>GPEFEAAACKKYMSKLRTIVAAQSRFLSTYDGAENLCLEDIYTENTLEVRTEVGMAGPLHKSPAALGLEELFSPNGHLNEDADTVLVVGEAGSGKSTLLQQVHLLWATGQDFQEFLFVFPFSCRQLQCVARPLSVMTLLFEHCCWPDVGQQDVFQFLLDHPDRILLTFDGFDEFKFKFTDHERHCSPTDPTSVQTLLFNLLQGNLLKNARKVLTSRPDAVSAFLRKYVRTEFNLKGFSEEGIELYLRKCHREPGVADRLIHLLQTTSALHGLCHLPVFSWMVSKCHQELLLQDGGSPKTTTDMYLLILQHFLRHASLPDSASQGLGPSLLQGRLPTLLRLGQLALWGLGMCCYVFSAQQLQAAQVDPDDISLGFLVQAQGVVPGSTAPLEFLHITFQCFLAAFYLVLSTDVPTASLRYLFNCRRPGSSPLSRLLPRLCVQGSEHKESTVAALLQKTEPHNLQITAAFLAGLLSREHRDLLAACQASERSLLRRRACARWCLARSLHKHFRSIPPAVPGEAKSMHAMPGFLWLIRSLYEMQEERLAQEAVRGLNVEHLKLTFCGVGPAECAALAFVLRHLRRPVALQLDHNSVGDIGVEQLLPCLGACKALYLRDNNISDRGICKLIEHALHCEQLQKLALFNNKLTDGCAHSVAQLLACKQNFLALRLGNNHITAEGAQVLAEGLRDNSSLQFLGFWGNKVGDKGAQALAEALSDHQSLKWLSLVGNNIGSVGAQALASMLEKNVALEELCLEENHLQDAGVCSLAEGLKRNSSLKVLKLSNNCITFVGAEALLQALASNDT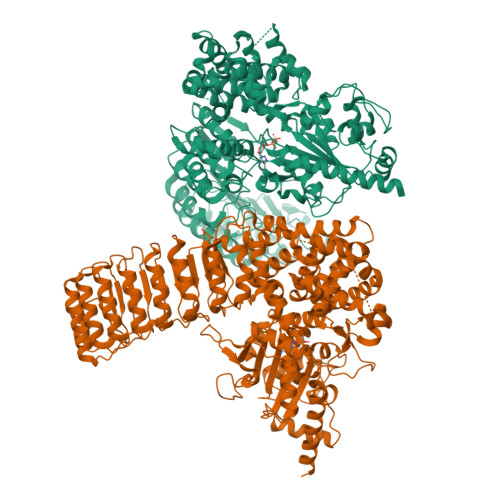ILEVWLRGNPFSPEEMEALSHRDSRLLL[2x]> MGNIMSASFAPECTDLKTKYDSCFNEWYSEKFLKGKSVENECSKQWYAYT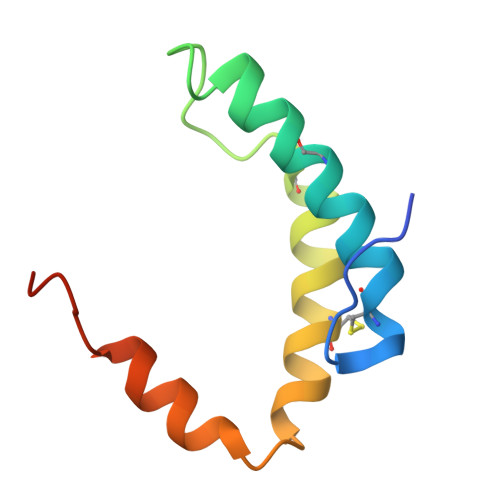TCVNAALVKQGIKPALDEAREEAPFENGGKL> DMRPEIRIAQ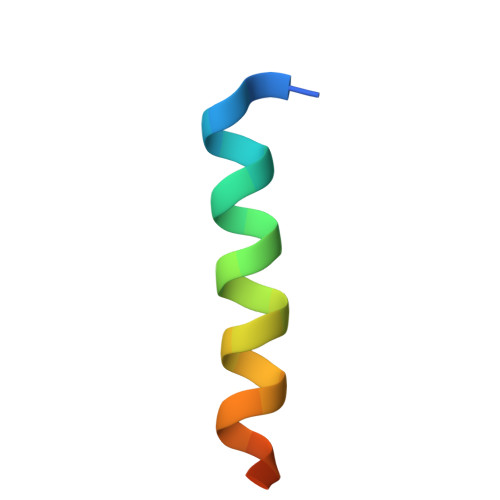ELRRXGDEFNATYARR3-[(3~{a}~{S},4~{S},6~{a}~{R})-4-carboxy-2,3,4,5,6,6~{a}-hexahydro-1~{H}-pyrrolo[2,3-c]pyrrol-3~{a}-yl]propyl-$l^{3}-oxidanyl-bis(oxidanyl)boranuide 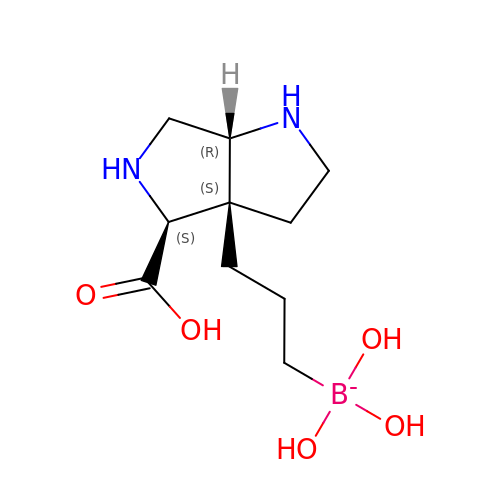| C10 H20 B N2 O5 | GRYGPEAWAXQHBS-XKSSXDPKSA-N O-phosphoseryl-tRNASec:selenocysteinyl-tRNASec synthase (SepSecS; SEPSECS) is an ubiquitously expressed enzyme that catalyzes the terminal reaction of selenocysteine synthesis. SepSecS converts the phosphoseryl (Sep) group into the selenocysteinyl (Sec) moiety in a mechanism that requires selenocysteine tRNA (tRNASec) and a pyridoxal-5-phosphate (PLP) cofactor. Previous structural work has shown that SepSecS is an obligate tetramer held by interactions between two homodimers. Recently, two research groups reported that four distinct mutations in human SEPSECS caused congenital cerebellar atrophy termed pontocerebellar hypoplasia type 2D (PCH2D).

To establish whether mutations T325S and Y334C alter the structure of SepSecS, we solved crystal structures of holo T325S and the T325S-tRNASec and Y334C-tRNASec complexes. The binary complex crystals belonged to the trigonal space group and contained two SepSecS dimers and one tRNASec molecule in the asymmetric unit, whereas those of the holo T325S were of the orthorhombic space group with half of the SepSecS tetramer in the asymmetric unit. On the other hand, Thr325 is located in helix α12 and ~15Å away from the active site. We hypothesized that the insertion of Ser in position 325 could introduce a kink in α12, thereby altering both the orientation of PLP and the overall conformation of the active site in human SepSecS4. A closer inspection of the crystal structure revealed that the Thr325 → Ser replacement does not cause any changes in the tetrameric structure of SepSecS. Based on the SAXS data, the T325S and Y334C mutations do not significantly alter the stoichiometry and architecture of the resulting binary complexes with tRNASec. A global structural comparison showed that T325S and Y334C tetramers adopt the same structure as the WT enzyme. We conclude that the Thr325Ser and Tyr334Cys mutations decrease the stability of SepSecS tetramers. In contrast, because only a small fraction of the T325S variant co-purifies with GroEL, it is likely the least damaging of the pathogenic variants.

>[4x]MNRESFAAGERLVSPAYVRQGCEARRSHEHLIRLLLEKGKCPENGWDESTLELFLHELAIMDSNNFLGNCGVGEREGRVASALVARRHYRFIHGIGRSGDISAVQPKAAGSSLLNKITNSLVLDIIKLAGVHTVANCFVVPMATGMSLTLCFLTLRHKRPKAKYIIWPRIDQKSCFKSMITAGFEPVVIENVLEGDELRTDLKAVEAKVQELGPDCILCIHSTTSCFAPRVPDRLEELAVICANYDIPHIVNNAYGVQSSKCMHLIQQGARVGRIDAFVQSLDKNFMVPVGGAIIAGFNDSFIQEISKMYPGRASASPSLDVLISLLSLGSNGYKKLLKERKEMFSYLSNQIKKLSEAYNERLLHTPHNPISLAMTLKTLDEHRDKAVTQLGSMLFTRQVSGARVVPLGSMQTVSGYTFRGFMSHTNNYPCAYLNAASAIGMKMQDVDLFIKRLDRCLKAVRKERSKESDDNYDKTEDVDIEEMALKLDNVLLDTYQDASS>QGMQYEWRKAELIGQLLNLGVTPGGVLLVHSSFRSVRPLEDGPLGLIEALRAALGPGGTLVMPSWSGLDDEPFDPATSPVTPDLGVVSDTFWRLPNVKRSAHPFAFAAAGPQAEQIISDPLPLPPHSPASPVARVHELDGQVLLLGVGHDANTTLHLAELMAKVPYGVPRHCTILQDGKLVRVDYLENDHCCERFA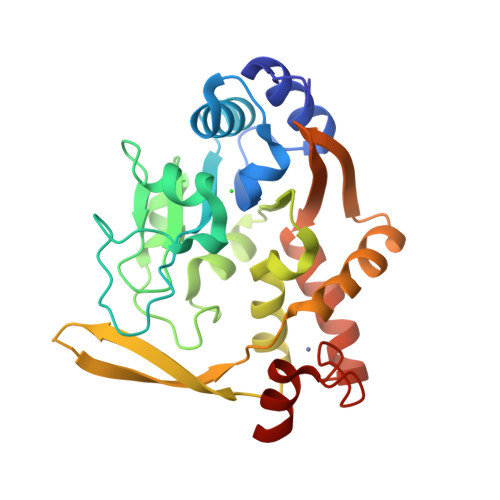LADRWLKEKSLQKEGPVGHAFARLIRSRDIVATALGQLGRDPLIFLHPPEAGCEECDAARQSIG[2x]> MPVDFTGYWKMLVNENFEEYLRALDVNVALRKIANLLKPDKEIVQDGDHMIIRTLSTFRNYIMDFQVGKEFEEDLTGIDDRKCMTTVSWDGDKLQCVQKGEKEGRGWTQWIEGDELHLEMRVEGVVCKQVFK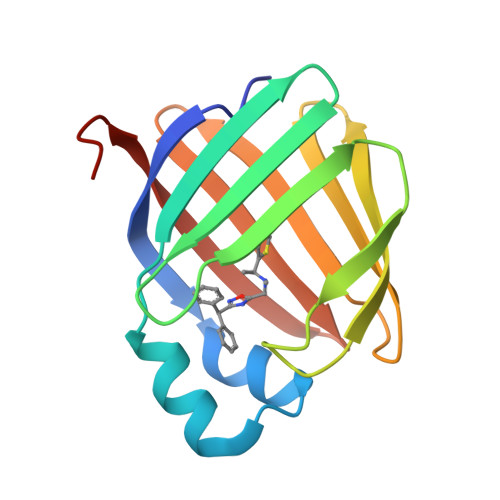KVQHHHHHH METHYL [(4S)-6-BROMO-2-METHYL-4-PHENYLQUINAZOLIN-3(4H)-YL]ACETATE | C18 H17 Br N2 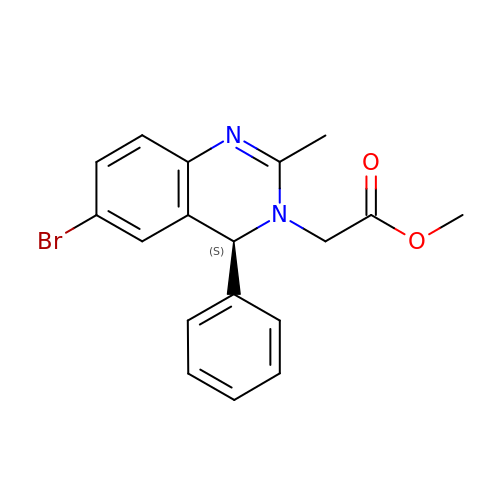O2 | ZWSKQYINLNUCMK-SFHVURJKSA-N The Escherichia coli CusA membrane protein, which recognizes and extrudes biocidal Cu(I) and Ag(I) ions, belongs to the heavy-metal efflux (HME) subfamily of RND efflux pumps. Typically, an RND efflux pump works in conjunction with a periplasmic membrane fusion protein and an outer membrane channel to form a functional tripartite protein complex. Extensive classification of the single-particle cryo-EM images of the CusA-Cu(I) complex revealed that there were four distinct populations of the CusA particles with different conformations that coexist in the nanodisc sample. Our data allow us to propose a simple model for the transport mechanism of the CusA HME-RND pump, where the CusA protomers can independently and uncoordinatedly function to export metal ion by progressing from the “binding” state to the “extrusion” state within the transport cycle.

The third most populated conformation of trimeric CusA in our cryo-EM sample has all three periplasmic clefts closed. We obtained 21,108 single-particle images for this conformation in our cryo-EM data set. The cryo-EM structure of this CusA trimer was solved to a resolution of 3.20 Å. Interestingly, the conformations of these three protomers are identical, presenting a symmetric, trimeric structure. The conformation of these three protomers is very similar to the conformation of the “extrusion” protomers of the EEB and EBB structures, with an “extrusion” channel observed to extend vertically through the periplasmic domain of each protomer with respect to the membrane surface. We, therefore, classify the conformational state of this symmetric trimer as the EEE form of CusA. To test the dynamics of the “extrusion” state of CusA, we added Cu(I) to the binding site in all three subunits of the EEE trimer. In these simulations, we observed transitions from the “extrusion” state toward the “binding” state. This transition is similar to that observed with the monomer simulation and occurs independent of the adjacent subunits.

>MGHHHHHHMIEWIIRRSVANRFLVLMGALFLSIWGTWTIINTPVDALPDLSDVQVIIKTSYPGQAPQIVENQVTYPLTTTMLSVPGAKTVRGFSQFGDSYVYVIFEDGTDPYWARSRVLEYLNQVQGKLPAGVSAELGPDATGVGWIYEYALVDRSGKHDLADLRSLQDWFLKYELKTIPDVAEVASVGGVVKEYQVVIDPQRLAQYGISLAEVKSALDASNQEAGGSSIELAEAEYMVRASGYLQTLDDFNHIVLKASENGVPVYLRDVAKVQIGPEMRRGIAELNGEGEVAGGVVILRSGKNAREVIAAVKDKLETLKSSLPEGVEIVTTYDRSQLIDRAIDNLSGKLLEEFIVVAVVCALFLWHVRSALVAIISLPLGLCIAFIVMHFQGLNANIMSLGGIAIAVGAMVDAAIVMIENAHKRLEEWQHQHPDATLDNKTRWQVITDASVEVGPALFISLLIITLSFIPIFTLEGQEGRLFGPLAFTKTYAMAGAALLAIVVIPILMGYWIRGKIPPESSNPLNRFLIRVYHPLLLKVLHWPKTTLLVAALSVLTVLWPLNKVGGEFLPQINEGDLLYMPSTLPGISAAEAASMLQKTDKLIMSVPEVARVFGKTGKAETATDSAPLEMVETTIQLKPQEQWRPGMTMDKIIEELDNTVRLPGLANLWVPPIRNRIDMLSTGIKSPIGIKVSGTVLADIDAMAEQIEEVARTVPGVASALAERLEGGRYINVEINREKAARYGMTVADVQLFVTSAVGGAMVGETVEGIARYPINLRYPQSWRDSPQALRQLPILTPMKQQITLADVADIKVSTGPSMLKTENARPTSWIYIDARDRDMVSVVHDLQKAIAEKVQLKPGTSVAFSGQFELLERANHKLKLMVPMTLMIIFVLLYLAFRRVGEALLIISSVPFALVGGIWLLWWMGFHLSVATGTGFIALAGVAAEFGVVMLMYLRHAIEAVPSLNNPQTFSEQKLDEALYHGAVLRVRPKAMTVAVIIAGLLPILWGTGAGSEVMSRIAAPMIGGMITAPLLSLFIIPAAYKLMWLHRHRVRK[3x]>[3x]GAPATVTEQGEDITSKKDRGVLKIVKRVGNGEETPMIGDKVYVHYKGK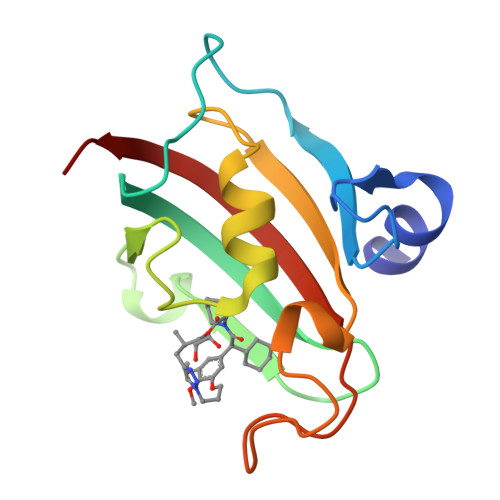LSNGKKFDSSHDRNEPFVFSLGKGQVIKAWDIGVATMKKGEIAHLLIKPEYAYGSAGSLPKIPSNATLFFEIELLDFKGE> MRFTFPLMAIVLEIAMIVLFGLFVEYETDQTVLEQLNITKPTDMGIFFELYPLFQDVHVMIFVGFGFLMTFLKKYGFSSVGINLLVAALGLQWGTIVQGILQSQGQKFNIGIKNMINADFSAATVLISFGAVLGKTSPTQMLIMTILEIVFFAHNEYLVSEIFKASDIGASMTIHAFGAYFGLAVAGILYRSGLRKGHENEESAYYSDLFAMIGTLFLWMFWPSFNSAIAEPGDKQCRAIVNTYFSLAACVL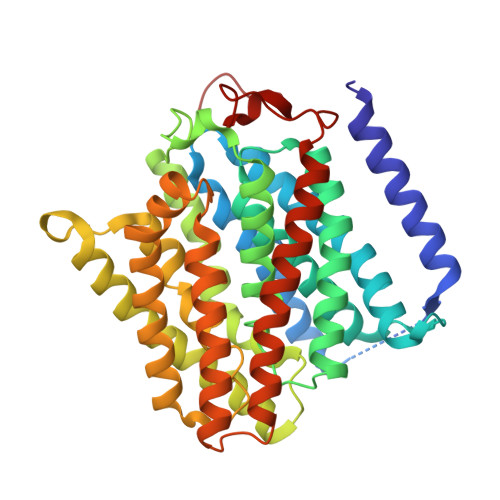TAFAFSSLVEHRGKLNMVHIQNATLAGGVAVGTCADMAIHPFGSMIIGSIAGMVSVLGYKFLTPLFTTKLRIHDTCGVHNLHGLPGVVGGLAGIVAVAMGASNTSMAMQAAALGSSIGTAVVGGLMTGLILKLPLWGQPSDQNCYDDSVYWKVPKTR> ELTPDQQTLLHFIMDSYNKQRMPQEITNKILKEEFSAEENFEILTEMATNHVQVLVEFTKKLPGFQTLDHEDQIALLKGSAVEA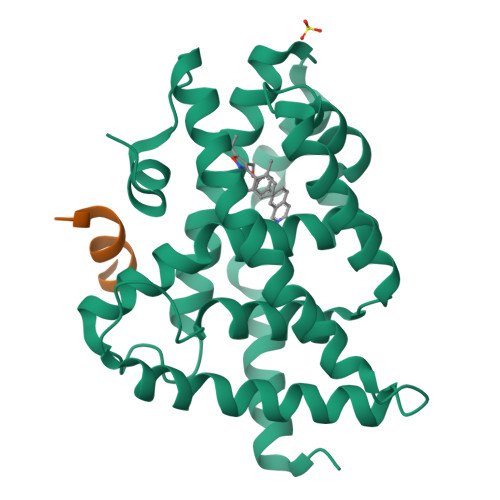MFLRSAEIFNKKLPSGHSDLLEERIRNSGISDEYITPMFSFYKSIGELKMTQEEYALLTAIVILSPDRQYIKDREAVEKLQEPLLDVLQKLCKIHQPENPQHFAELLGRLTELRTFNHHHAEMLMSWRVNDHKFTPLLEEIWDVQ;> DHQLLRYLLDK> HHHHHHSSGMASINLPFSLSGSKRIPTSEELADGYQCGPLDVELDNWLMWWLTGQVDGVIEGAGLT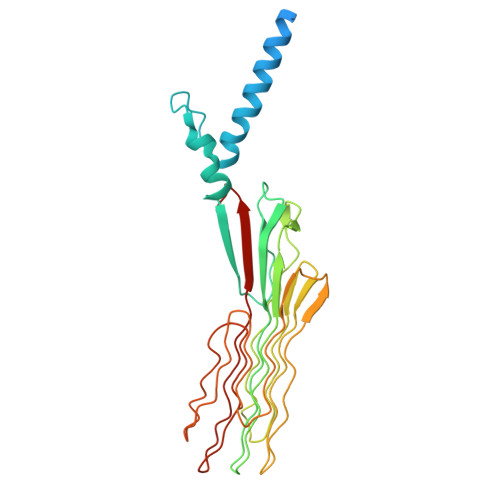TDDTDLARLYKAIQSMTSGNLRTVVLTAASGNLPIPSDVSVLNWVRAVGGGGAGGNSNTGNSKASGGGGGAGFDRFNVAVTPGSNVPYTVGAAGAVNGLGAGYNGGAGGSTAILGTTAGGGAGGLGVNNNATAVQVNGGTTSGTTPEISYPGGLGTEGIVGTGGGSVLSQPTQRAFTNAGNNNPANSWGGGGPGGSDFGGAWQPGGVGKQGIIIVQYFSRFAP>MRGSHHHHHHGSVTCTGCVDLDELSFEKTVERFPYSVVKFDIAFPYGEKHEAFTAFSKSAHKATKDLLIATVGVKDYGELENKALGDRYKVDDKNFPSIFLFKGNADEYVQLPSHVDVTLDNLKAFVSANTPLYIGRDGCIKEFNEVLKNYANIPDAEQLKLIEKLQAKQEQLTDPEQ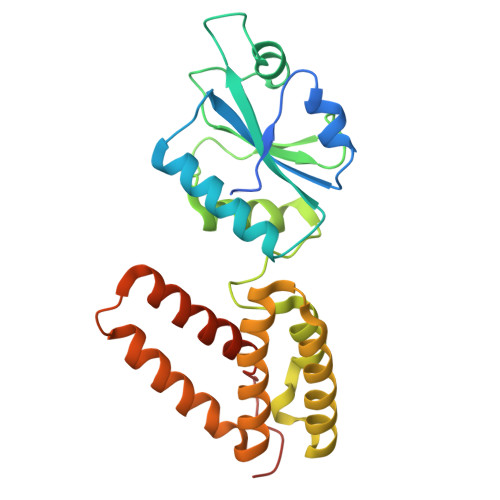QQNARAYLIYMRKIHEVGYDFLEEETKRLLRLKAGKVTEAKKEELLRKLNILEVFRVHKVTKTAPEKEEL[2x]2'-FLUOROGUANYLYL-(3'-5')-PHOSPHOCYTIDINE 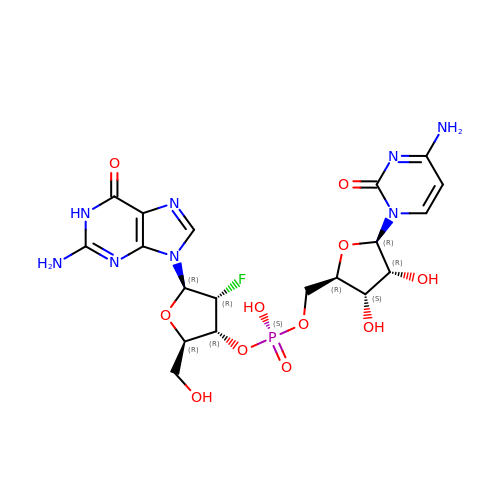| C19 H24 F N8 O11 P | ZSBUMMSBXYRQAK-FOJQSULLSA-N>MEDAKNIKKGPAPFYPLEDGTAGEQLHKAMKRYALVPGTIAFTDAHIEVNITYAEYFEMSVRLAEAMKRYGLNTNHRIVVCSENSLQFFMPVLGALFIGVAVAPANDIYNERELLNSMNISQPTVVFVSKKGLQKILNVQKKLPIIQKIIIMDSKTDYQGFQSMYTFVTSHLPPGFNEYDFVPESFDRDKTIALIMNSSGSTGLPKGVALPHRTACVRFSHARDPIFGNQIIPDTAILSVVPFHHGFGMFTTLGYLICGFRVVLMYRFEEELFLRSLQDYKIQTALLVPTLFSFFAKSTLIDKYDLSNLHEIASGGAPLSKEVGEAVAKRFHLPGIRQGYGLTETTSAILITPEGDDKPGAVGKVVPFFEAKVVDLDTGKTLGVNQRGELCVRGPMIMSGYVNNPEATNALIDKDGWLHSGDIAYW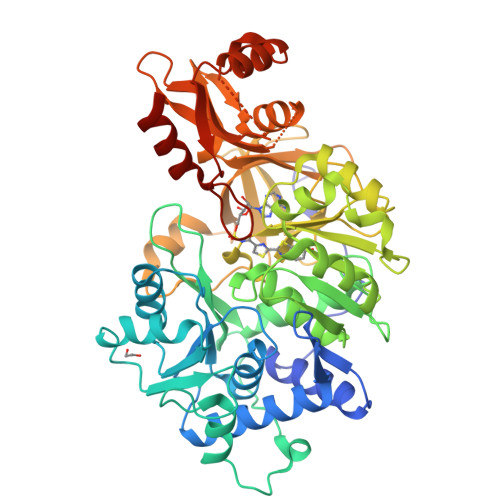DEDEHFFIVDRLKSLIKYKGYQVAPAELESILLQHPNIFDAGVAGLPDDDAGELPAAVVVLEHGKTMTEKEIVDYVASQVTTAKKLRGGVVFVDEVPKGLTGKLDARKIREILIKAKKGGKSKL[2x]> XMKQYLEL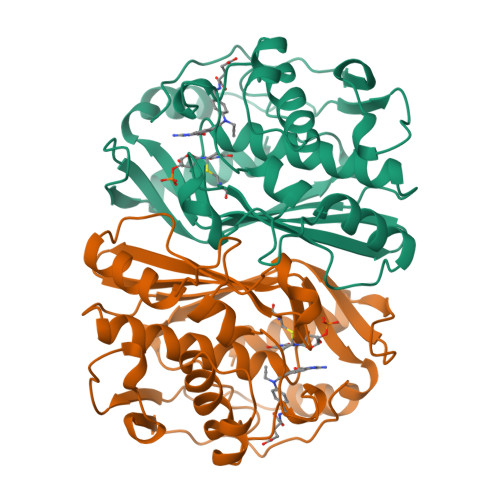MQKVLDEGTQKNDRTGTGTLSIFGHQMRFNLQDGFPLVTTKRCHLRSIIHELLWFLQGDTNIAYLHENNVTIWDEWADENGDLGPVYGKQWRAWPTPDGRHIDQITTVLNQLKNDPDSRRIIVSAWNVGELDKMALAPCHAFFQFYVADGKLSCQLYQRSCDVFLGLPFNIASYALLVHMMAQQCDLEVGDFVWTGGDTHLYSNHMDQTHLQLSREPRPLPKLIIKRKPESIFDYRFEDFEIEGYDPHPGIKAPVAI>[2x]AYAQWVIIIIHNVGSKDVKIKNLKPSWGKLHADGDKDTEVSASKYEGTVIKPDEKLQINACGRSDAAEGTTGTFDLVDPADGDKQVRHFYWDCPWGSKTNTWTVSGSNTKWMIEYSGQNLDSGALGTITVDTLKK;> SQAGDTLNDVIQDPTRRNKLINDNNLLKGIIMGRDGPVPSSRELIVRPDTLRAIINNRATIETTTMKSMYTSSRYLFPQGRIDFTTPDSGFDDVIKLSPQFTSGVQAALAKATGTEKREALQNLFQEYGHVFRTKVHIGGVLSAHTMETFSKLNVKYIVNGGDYTKIQNTEEWVASTNQSEHWRVIEVTEVTAVADLLPQPIRGQVK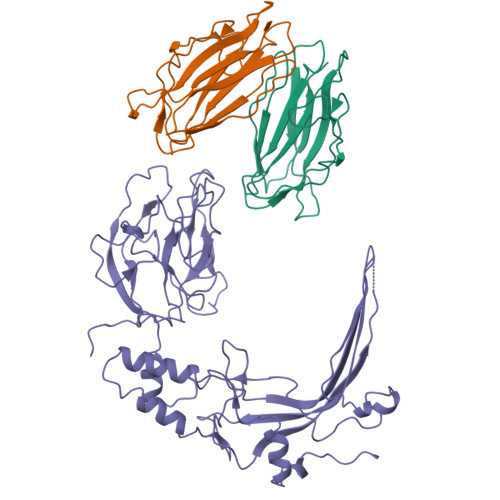DLLKPLLGKWVDVEKVPGLESLPVSVYRPKGAIPAGWFWLGDTADASKALLVKPTLPARSGRNPALTSLHQGSGMTEQPFVDLPQYQYLSTYFGSFAHDTPPGSTLRGLRPDHVLPGRYEMHGDTISTAVYVTRPVDVPFPEDECFDLKSLVRVKLPGSGNPPKPRSALKKSMVLFDSGEK>AFAKVTMLYVPCTINQVLVKAFVDSGAQNSIMNKRTAERCGLMRLVDVRMRGVAVGVGRQEICGRIHMTPVNLAGMYIPFAFYVIEDQAMDLIIGLDQLKRHQMMIDLKHNCLTIDNINVPFLPENDLPA[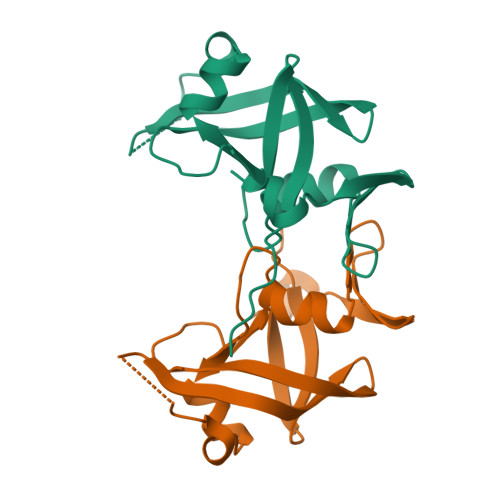6x]> CASHNENASLLAKKQAQNISQNLPIKSAG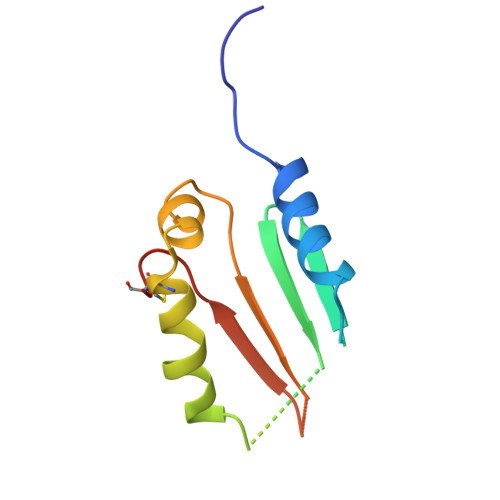YTLVLAQSSGTTVKMTIISEAGTQTTQTPDAFLTSYQRQMCADPTVKLMLTEGINYSITINDTRTGNQYQRKLDRTTCGIVKA> MWSHPQFEKENLYFQGIYISAVGMLNALGDNVDDIAQNLVLGQAPGMYERSGWLQPGKTCCLGGVDAELPAMPDMLSEHNSRNNRLLLAALMQIKPQVDEAIARHGRERIAVIMGTSTSGLDEGDQHVSRTVYQQSHGSYHDYHYYQQELGDPSRFLARYLAIEGPAFTLSTACSSSSRAIISGQRLIEMGLVDAAIVGGADTLSRMPINGFDSLESLSPTLCEPFCQDRQGITIGEASTLLLLTREPQPIALLGVGESSDAWHMSAPHPEGRGAIAAINMALRKAGISPAEIGYINLHGTGTKLNDQMESIVINQIFGENTPCSSTKYLTGHTLGAAGACEAGLCWLLLTRHLPLPAQDFTRSGIDIALPACGLLTQSQPLEKPIVMSNSFAFGGNNTSLILGVA;> MKLTLDITDWQAIAPGLSLTEEWKAWSATLPAAIDKSRPLEKCTQLPMMTARRLSSGSRLAVDCGLSLLRRHQVDAIVYTSRHGELERNYQILQNLAQQESISPTNFAMSVHNSSVGNLTIVAKAPLVSSSVSAGIDSFQQGLFEALTLIH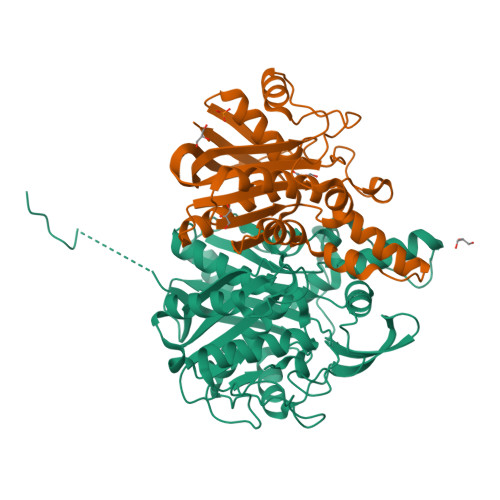AGHRKVLFVDFEGEIPGFYHNVIDAKTPTYPFAVALLLEQGAGLSCTKQSSMETEPSLPQSLQFLHGWLRGEQHFVVSGDHCQWNWSR>[2x]VGSLNCIVAVSQNMGIGKNGDLPWPPLRNEFRYFQRMTTTSSVEGKQNLVIMGKKTWFSIPEKNRPLKGRINLVLS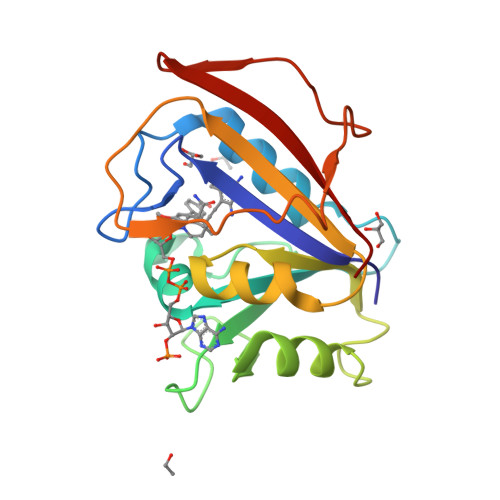RELKEPPQGAHFLSRSLDDALKLTEQPELANKVDMVWIVGGSSVYKEAMNHPGHLKLFVTRIMQDFESDTFFPEIDLEKYKLLPEYPGVLSDVQEEKGIKYKFEVYEKND>[4x]GAMASGKVVKFSYMWTINNFSFCREEMGEVIKSSTFSSGANDKLKWCLRVNPKGLDEESKDYLSLYLLLVSCPKSEVRAKFKFSILNAKGEETKAMESQRAYRFVQG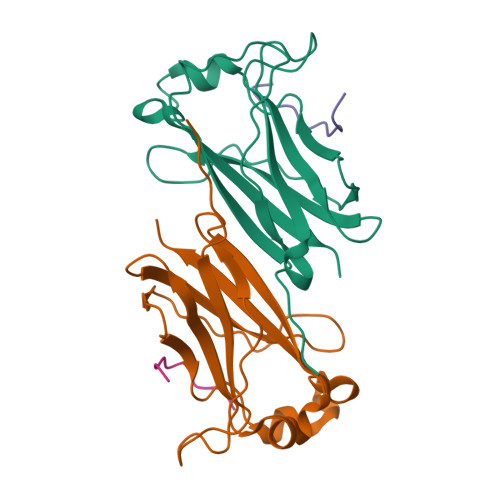KDWGFKKFIRRDFLLDEANGLLPDDKLTLFCEVSVVQD;>[4x]EPEQDSAVTSGE> MSNVPAELKY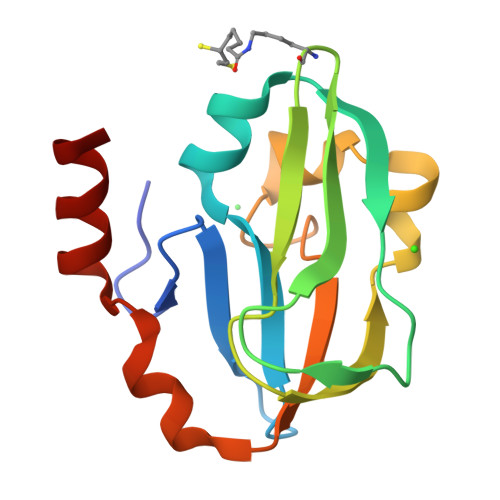SKEHEWLRKEADGTYTVGITEHAQELLGDMVFVDLPEVGATVSAGDDCAVAESVKAASDIYAPVSGEIVAVNDALSDSPELVNSEPYAGGWIFKIKASDESELESLLDATAYEALLEDE> NECLGTIGPVTPLDASDFALDIRMPGVTPKESDTYFCMSMRLPVDEEAFVIDFKPRASMDTVHAMLLFGCNMPSSTGSYWFCDEGTCTDKANILYAWARNAPPTRLPKGVGFRVGGE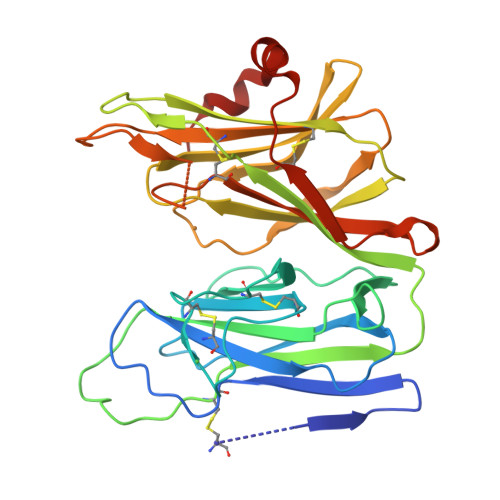TGSKYFVLQVHYGDISAFRDNHKDCSGVSVHLTRVPQPLIAGMYLMMSVDTVIPPGEKVVNADISCQYKMYPMHVFAYRVHTHHLGKVVSGYRVRNGQWTLIGRQNPQLPQAFYPVEHPVDVTFGDILAARCVFTGEGRTEATHIGGTSSDEMCNLYIMYYMEAKYALSFMTCTKNVAPDMFRTIPAEANIPIPV> ACR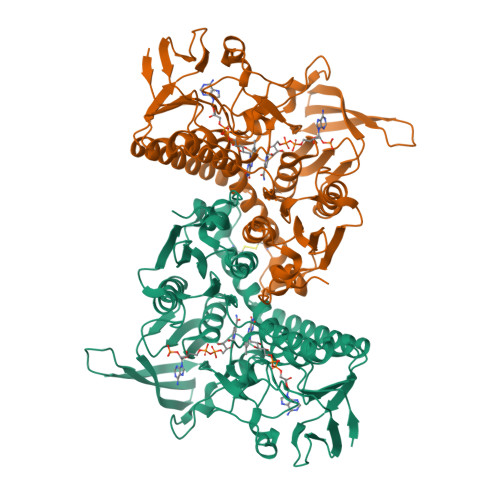QEPQPQGPPPAAGVASYDYLVIGGGSGGLASARRAAELGARAAVVESHKLGGTCVNVGCVPKKVMWNTAVHSEFMHDHADYGFPSCEGKFNWRVIKEKRDAYVSRLNAIYQNNLTKSHIEIIRGHAAFTSDPKPTIEVSGKKYTAPHILIATGGMPSTPHESQIPGASLGITSDGFFQLEELPGRSVIVGAGYIAVEMAGILSALGSKTSLMIRHDKVLRSFDSMISTNCTEELENAGVEVLKFSQVKEVKKTLSGLEVSMVTAVPGRLPVMTMIPDVDCLLWAIGRVPNTKDLSLNKLGIQTDDKGHIIVDEFQNTNVKGIYAVGDVCGKALLTPVAIAAGRKLAHRLFEYKEDSKLDYNNIPTVVFSHPPIGTVGLTEDEAIHKYGIENVKTYSTSFTPMYHAVTKRKTKCVMKMVCANKEEKVVGIHMQGLGCDEMLQGFAVAVKMGATKADFDNTVAIHPTSSEELVTLR methyl (2~{R})-2-[(4~{S})-6-(4-chlorophenyl)-8-methoxy-1-methyl-4~{H}-[1,2,4]triazolo[4,3-a][1,4]benzodiazepin-4-yl]pent-4-enoate 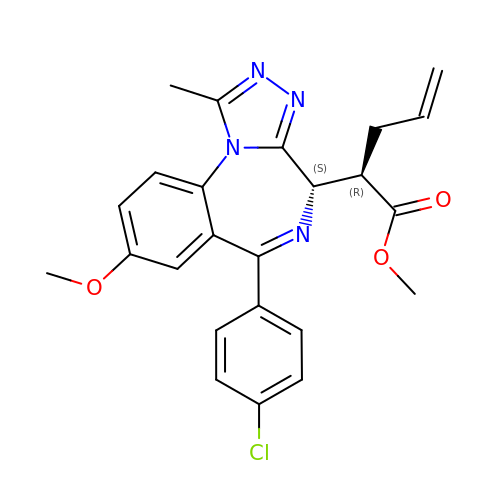| C24 H23 Cl N4 O3 | LNODZYMQLCXVKL-GCJKJVERSA-N>[2x]MSLPML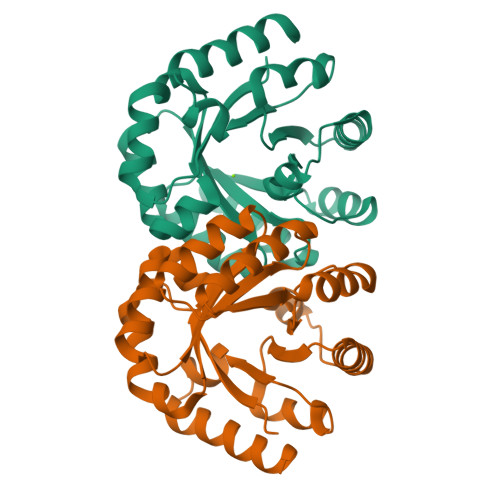QVALDNQTMDSAYETTRLIAEEVDIIEVGTILCVGEGVRAVRDLKALYPHKIVLADAKIADAGKILSRMCFEANADWVTVICCADINTAKGALDVAKEFNGDVQIDLTGYWTWEQAQQWRDAGIGQVVYHRSRDAQAAGVAWGEADITAIKRLSDMGFKVTVAGGLALEDLPLFKGIPIHVFIAGRSIRDAASPVEAARQFKRSIAELWG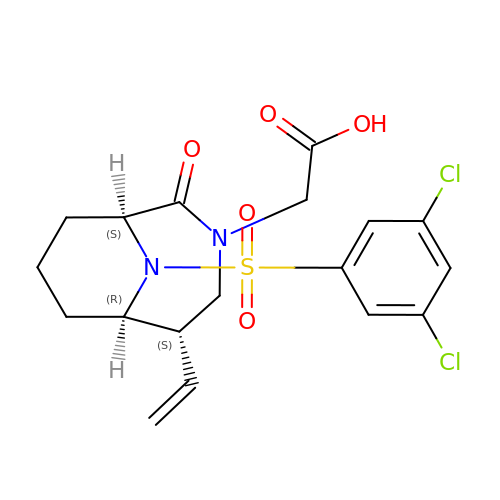2-[(1~{S},5~{S},6~{R})-10-[3,5-bis(chloranyl)phenyl]sulfonyl-5-ethenyl-2-oxidanylidene-3,10-diazabicyclo[4.3.1]decan-3-yl]ethanoic acid | C18 H20 Cl2 N2 O5 S | CWGQECKQFWBWHJ-XZJROXQQSA-N>SNAEARGFTAEDFALSHPGGALGRKLLLRVNDIMHTGDEIPHVGLQATLRDALLEITRKNLGMTAICDDDMNIIGIFTDGDLRRVFDTGVDMRDASIADVMTRGGIRIRPGTLAVDALNLMQSRHITCVLV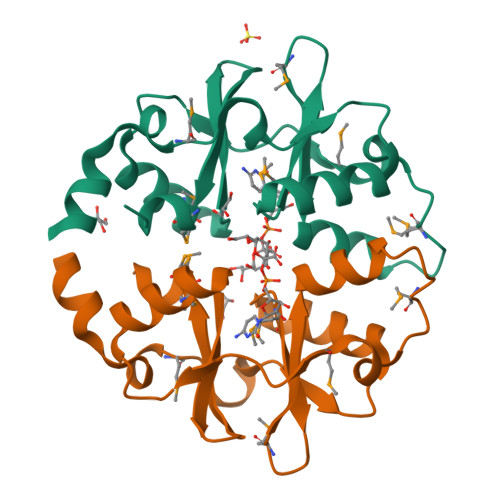ADGDHLLGVVHMHDLLRA[2x]> SHHHHHHMGWDLTVKMLAGNEFQVSLSSSMSVSELKAQITQKIGVHAFQQRLAVHPSGVALQDRVPLASQGLGPGSTVLLVVDKCDEPLSILVRNNKGRSSTYEVRLTQTVAHLKQQVSGLEGVQDDLFWLTFEGKPL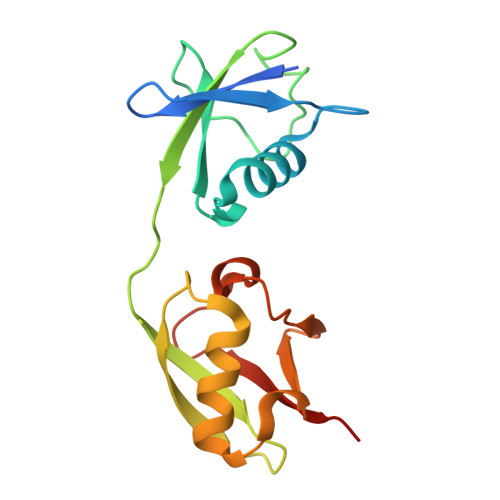EDQLPLGEYGLKPLSTVFMNLRLRGG>[3x]MPEGADPVAEVKTALAGFLKEVKGFQDDVKTRLQQQEERVTMLQTKTYAGRHALAAAATEEAPHQKAFAAYLRTGDDDGLRGLSLEGKALNSAVAAEGGYLVDPQTSETIRGVLRSTASLRQIASVVNVEATSFDVLVDKTDMGSGWASETAALSETATPQIDRITIPLHELAAMPKASQRLLDDSAFDIETWLANRIADKFARAEAAAFISGDGVDKPTGFLTKTKVANGAWA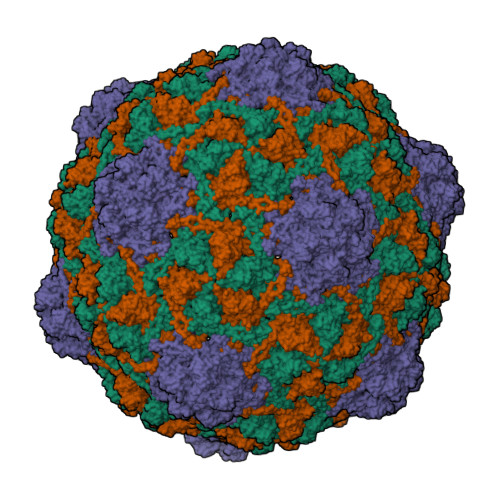WGSLGYVATGAAGDFAAVNASDAVVDLVYALGAEYRANASFVMNSKTAGAVRKMKDADGRFLWADSLAAGEPARLMGYPVLIAEDMPDIAANAYAIAFGDFGNGYTIAERPDLRVLRDPFSAKPHVLFYASKRVGGDVSDFAAIKLLKFAAS> ALSKVVIRRLPPTLT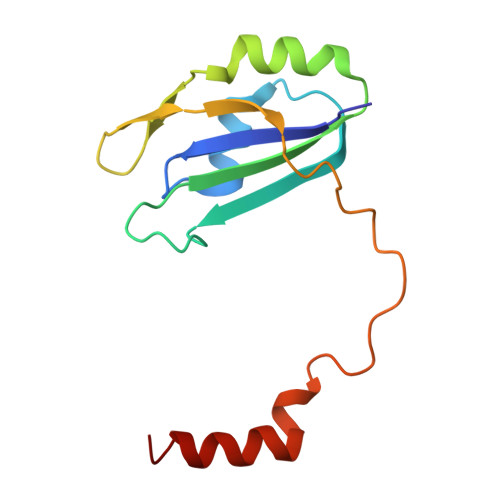KEQLQEHLQPMPEHDYFEFFSNDTSLYPHMYARAYINFKNQEDIILFRDRFDGYVFLDNKGQEYPAIVEFAPFQKAAKKKTKKRDTKVGTIDDDPEYRKFLESYATD>MHHHHHHANVTSIRTEPTYTLYATFDNIGGLKARSPVSIGGVVVGRVADITLDPKTYLPRVTLEIEQRYNHIPDTSSLSIRTSGLLGEQYLALNVGFEDPELGTAILKDGDTIQDTKSAMVLEDLIGQFLYGSKGDDNKNSGDAPAAAPGNNETTEPVGTTK[3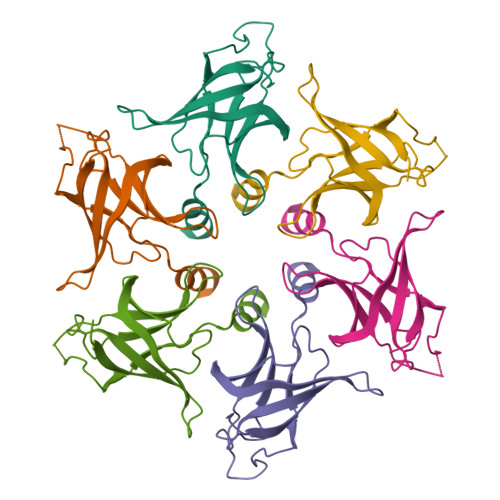x]Dictyostelium myosin-II heavy chain kinase A (MHCK-A) phosphorylates the α-helical coiled-coil tail of myosin-II, causing contractile bipolar filaments of myosin-II to disassemble into inactive monomers. MHCK-A is a member of the atypical α-kinase family of serine/threonine protein kinases. The α-kinase domain is bi-lobed, with the active site located in a large cleft at the junction of the two lobes. The α-kinase N-lobe is similar to the N-lobe of other protein kinases but the C-lobe has a distinctive structure and requires a tightly bound zinc atom for stability.

To gain further insight into the function of Asp663, an A-CAT D663A mutant was crystallized and its structure was solved to a resolution of 2.5 Å. Although A-CAT-D663A was crystallized in the presence of MgATP, AMP was present in the catalytic cleft. Asp766 was not phosphorylated in the A-CAT-D663A structure. A surface representation of A-CAT-D663A shows that the left-hand side of the catalytic cleft is closed whereas the right-hand side is open. The D663A mutation eliminates a hydrogen bond interaction between Asp663 and the Tyr647 residue located at the end of the β7 strand. The hydrogen bond with Asp663 attracts Tyr647 towards the C-lobe, so that it can interact with Leu659 in the αC helix, which in turn interacts with Leu779 in the N/D-loop. The absence of the hydrogen bond in A-CAT-D663A causes Tyr647 to move upwards by 1.8 Å. The upwards movement is transmitted to the adjacent β6 strand and P-loop and disrupts the hydrophobic interaction with Leu659, causing the side chains of Leu659 and Leu759 to moves outwards by 3.0 Å. A-CAT-D663A retains the ability to hydrolyze ATP and ADP, showing that Asp663 is not essential for catalytic activity. The D663A and D663S mutants retained between 25 and 50% of wild-type ATPase activity, but exhibited extremely low kinase activity (~1% of wild-type).

>MGGHHHHHHGENLYFQGISSETGEMGILWEFDPIINKWIRLSMKLKVERKPFAEGALREAYHTVSLGVGTDENYPLGTTTKLFPPIEMISPISKNNEAMTQLKNGTKFVLKLYKKEAEQQASRELYFEAVKMQMVCRDWGNKFNQKKPPKKIEFLMSWVVELIDRSPSSNGQPILCSIEPLLVGEFKKNNSNYGAVLTNRSTPQAFSHFTYELSNKQMIVVDIQGVDDLYTDPQIHTPDGKGFGLGNLGKAGINKFITTHKCNAVCALLDLDVKLGGVLSGNNNQQLQQGTMVKADILPELMPSDNT[2x]> RSLLKTKENLGSGFISLFRGKKIDDDLFEELEEQLLIADVGVETTRKIITNLTEGASRKQLRDAEALYGLLKEEMGEILAKVDEPLNVEGKAPFVILMVGVNGVGKTTT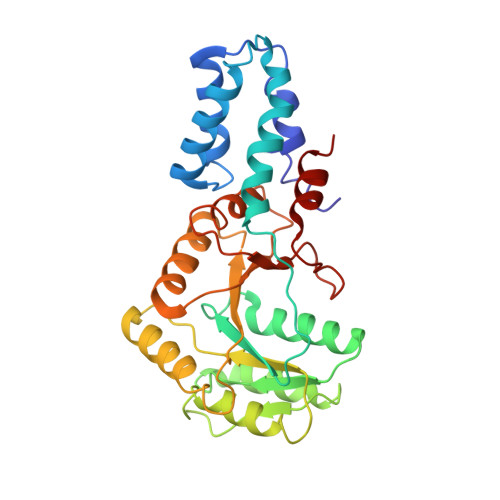IGKLARQFEQQGKSVMLAAGDTFRAAAVEQLQVWGQRNNIPVIAQHTGADSASVIFDAIQAAKARNIDVLIADTAGRLQNKSHLMEELKKIVRVMKKLDVEAPHEVMLTIDASTGQNAVSQAKLFHEAVGLTGITLTKLDGTAKGGVIFSVADQFGIPIRYIGVGERIEDLRPFKADDFIEALFAR> MKFGNFLLTYQPPELSQTEVMKRLVNLGKASEGCGFDTVWLLEHHFTEFGLLGNPYVAAAHLLGATETLNVGTAAIVLPTAHPVRQAEDVNLLDQMSKGRFRFGICRGLYDKDFRVFGTDMDNSRALMDCWYDLMKEGFNEGYIAADNEHIKFPKIQLNPSAYTQGGAPVYVVAESASTTEWAAERGLPMILSWIINTHEKKAQLDLYNEVATEHGYDVTKIDHCLSY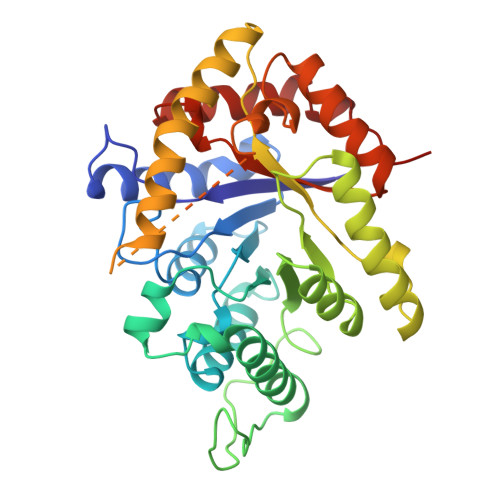ITSVDHDSNRAKDICRNFLGHWYDSYVNATKIFDDSDQTKGYDFNKGQWRDFVLKGHKDTNRRIDYSYEINPVGTPEECIAIIQQDIDATGIDNICCGFEANGSEEEIIASMKLFQSDVMPYLKEKQ> SDAEKVYDIEGYPVFLGSEYYIVSAIIGAGGGGVRPGR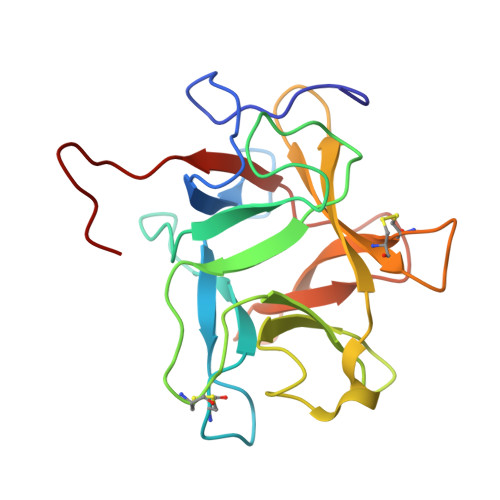TRGSMCPMSIIQEQSDLQMGLPVRFSSPEEKQGKIYTDTELEIEFVEKPDCAESSKWVIVKDSGEARVAIGGSEDHPQGELVRGFFKIEKLGSLAYKLVFCPKSDSGSCSDIGINYEGRRSLVLKSSDDVPFRVVFVKPRSGSETES Here, we show that dipeptidyl peptidase 11 (DPP11), a central metabolic enzyme in these bacteria, undergoes a conformational change upon peptide binding to distinguish substrates from end products. As previously reported, the overall fold of DPP11 comprises a bilobal architecture. The upper helical domain dictates the specificity of the enzyme and caps the catalytic domain, which has a typical chymotrypsin double β-barrel fold. The active site of DPP11 lays in a wide cleft running through the middle of the protein between the catalytic and helical domains, which contributes to the formation of the substrate binding subsites.

We determined the structures for the inactive constructs PgDPP1122-720 S655A, PeDPP1122-717 S652A and its complexes with the dipeptides Arg-Asp and Arg-Glu, as well as the substrate Leu-Asp-Val-Trp, at 2.4, 2.85, 2.2, 2.1 and 2.6 Å resolution, referred to as PgDPP11, PeDPP11, PeDPP11:RD, PeDPP11:RE and PeDPP11:LDVWs, respectively. PeDPP11 and PgDPP11 superposition yielded a root mean square deviation (r.m.s.d.) of 1.4 Å for 629 out of 685 superimposed Cα-atoms. The binding of peptides to PgDPP11 induces the dimerization of its monomeric population, masking the real thermodynamic contributions involved in the binding process. In this way, we focused our thermodynamic analysis solely on PeDPP11. Indeed, P. gingivalis dpp11-knock-out strain shows growth impairment, suggesting its critical role in the bacterium energy metabolism.

>[2x]MDEGMWLMQQLGRKYAQMKERGLKMKEYDLYNPNGTSLKDAVVLFDGGCTGEVVSDRGLVLTNHHCGYDMIQAHSTLEHNYLENGFWAMREADELPNKDISVVFIDKIEDVTDYVKKELKAIKDPNSMDYLSPKYLQKLADKKAGKNFSAKNPGLSVEIKAFYGGNLYLMFTKKTYTDVRLVGAPPSSIGKFGADTDNWIWPRHTGDFSIFRIYADKNGNPAPYSEDNVPLKPKRFFNISLGGVQENDYAMIMGFPGTTHRYFTASEVDEWKSIDNDIRIRMRDIRQGVMLREMLADPQIKIMYSAKYAASQNAYKRAIGANWAIKTRGLRQNKQAMQDRLIAWGAKQGTPRYEEAVHEIDATVAKRADLRRRYWMIEEGIIRGIEFARSPIPTEDETKALQGNDASARKEAIDKIRTRYSKFANKDYSAEVDKKVAVAMLTEYLKEIPYENLPLHLRLVKDRFAGDVQAYVDDIFARSVFGSEAQFDAFAAVPSVEKLAEDPMVLFASSVFDEYRKLYNELRPYDDPILRAQRTYIAGLLEMDGDQDQFPDANLTLRFTYGQVKGYSPRDNVYYGHQTTLDGVMEKEDPDNWEFVVDPKLKAVYERKDFGRYADRSGRMPVAFCATTHTTGGNAGSPVMNANGELIGLNFDRNWEGVGGDIQYLADYQRSIIVDIRYVLLVIDKVGGCQRLLDEMNIVPHHHHHH>MAATRQIQYTIPPREDYNKLSDEQKTRISEAFELFDSNKDGLLSYEEFRFVLRALGFDLPKQQTYDMLVRHGQRPANWPHDQECPPVYRQFNLATAQALAGTLIRQRDPRDELRRAFRLFDVDGKGMITEDDLRKVCQQVGNNIPDADIQAMIEEFDSNGKGGVDEDEFLRLMMSKK[2x];>[2x]GHMKPKRDLMADFTKWFVTGDGGIMEEFTEETLRHLLWDVWQRHQREEAERKRKAEEEESWRLAREHLTHRLQVKYFYRWREKARALAT;>[2x]GSSHHHHHHSQDLMASQHSPTPVKVPAAAANYTPATLDQDLRSQINSLLIKEGHVAKIQEHLLHHLHAHPSNWPTVVQNHALSLLRSGEVTSFPALLRRVVEDVRQDTALAPSSTTANGNGESTTTNGATNGKGATTN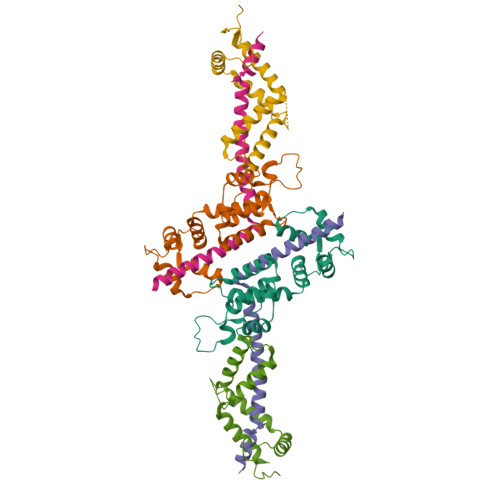GNKGGVADLKPSLAVPQSVVEEALKVTRECLDQLCEIEEPLAA>GSTANKLTEAQRRIAELEKELQRTTQRVDQLSDVVQQQKDELQAAKDRHALEMEETRHAYNAVIHRKDEVQEEALRQLLKSRQLMVSAARYEAVVAAKKLHAQEFELGAPAGRQACGRIML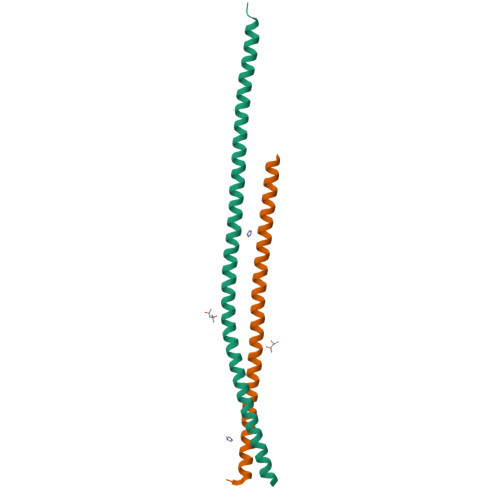KSNRK[2x]>[2x]MKKQKRTQGKQNTKQIKQEKLSSKRKANNQKEGKKKVKQEDYKEIKQKGKRMLSKIVKASFSSKGFNLANAVNTVKSTLNAPIKHIKRNIEPTGSNYSRMTNTTEEAFDEVSHEWQALVTSNPFDLNVFNYLENTQTSNFGTVDNPLVVFTSETPFRYVGCTGQMNEDDYEGHELLFFLLREGSLQRCMGCGQVFKLVRLRNEYSPEMDYYLSNFHPYEMQEMGESDTTVLMSPYKYASHYEYTQFETPSNMVYSMVNPDEHDRLLVDPAYRMERTKALEEKYKVYTSSLREVEKQFEERYGRAGQINISKVTYSTLIDVEKAVLKMDRLFRKVAKFENRAFIDRANHSRREKRMLERAQQRWDSNYSFFTGSLTEEEQKYRDYYETELEAYPEDEGIEQQLDQQEVLLSGRYDPKLYDFQEGYTKNPEDDQTSLIEKKAFKFRYRLANETSETFQRRNNRMVERQIKRFQQPQYKHAFEQLQKNIAISSNSGNALHSEYGYLELLSNESVQLYKDYYESDAEEDFKVFENLSSKEKLVMIANFENNLLPKYDRSEVHLIPKRQWEPAFGVWENFLYDITEYASFIAPRGKEIAADYQIQSAIPLTKEELIEAGLYKETIEKKVEPKLEAKKQTKSE;>MIWKYLQRTNRGNIIQAGLQHRKFENLPFKQNFDNLTKAYDLRMWYISNSPHEAKNLEYVNELEALHNELNYQNSRQFLFRTVSFLLGWALFYQFYELPKTYDWQDTQEPKHQVPAYGDLEEGGDEGGDD[2x];>MSSAVEKKDLPADYGKMPAGYNFLTRGKDWREYDKDFILRTDAVWEKFQLEHFFRNYMKCFFFDHGLKKYQMFEPEDMYTVVFEGWALDDLITFPGFTPTGRTNSYQIGLSPRQRTVVPTQTFYQMQDYYMLCGLRFERWFRCDLVYHDQRHTKFDQVKNQKNYKTYPCYREYYEAQYACQDDMFDFLMELAYARRAADNFESDFASHELTTLPTFYDTPKAAERKTYTY[2x];>MGSVWFRNRYWWYRSLYDDYVAREAKLAFGIAAFIWLPHYYWGIHLNRAFEVNFSHRNYAHEWGPRRNRLAHSLEFEQFDMILENWQDLEDEYAQRGDGMLKK[2x];>MEVKYRGPSDDKLECEFLENNLLSCLREKSVQDNVAKMTCRPEFLVWFFLECPTKAAVYHDPKGLRNIFIQDKIKQKGSDDGVLSKDD[2x];>[2x]MNRFFKVSSKYQYYKYLEQYDAAFLRKYQSETHWYLGRRGAWKNLVIKYAGDHISLEEEHNVKYKTHLSFVYLSYRLAWVLFAYVLIYNHFLLGDIGKTFNVGEWDHRLKPSAERDYPTRYESLYILDRTQKW;>MISKYRYLHCARKLVKQSVQAFGGGHHHHEYDWRDDPKVNKDIEEDIRDRGWHPETYDFPYTKKHDDWVFDVTMPSQNYQTDLTVNIHPENKKMHVMKQVMRQSYWDAEHDMAHEYDYESEDLDFQCESFKSQHFRKKGPISQYLILGLLPILYFGTEFFYNHYPDEDYWRVAHPPPLDYPDTDDTDDTETFKDYKSFTGRRMVDTGIVDPLWYDIREGKKVYYDWAGVNQPMEDI[2x];>MNKSQDEVKEDYFSIKKKKYNSLDCVLSPIVTRKKQESINSFQAGLQEDQNSTAVPESPFIRNCSETLNRSQHKILDHYFEYDYSLKKKIEKIKISLQNKTGTDSSQSLVQKRLDDLRKKTLIYKQFNIQKNNNNINNTGQFFIEKDKQNNLNLSQPHQIIKSKQGHKRSFTNTLYCSSNDKKIFNISSQKQNIKTVKQSNNSSMYEEQIKNDQNKKQNFNKQAKSERKQAEFCDLFYESMQKDAERQFKSNSDKSKSITQILENNCENAIVLLNHLIQILTDSIPISKNSILLDEKLSQCVNLSNNSKISQLMLVIQKLQGKISYYYNDFLKCIRMMKICKNFCQLFGTLKFKISCYKYIGLGFQRLNKPKVALVYFVKMLRQSWFLKQEDQEINSYDFIGMSYFYLGSIDKAYQYHQMMIDGIKADEEVKKISNIMLKNRKYSNYPTLQNIRIIQETSDGQPLQKTIRKSKIINPQFQLTQQEWGENISSSEDEFELPQMQIAVKNAEEQTFQKKFLSTPWNDRFIQAQIHKLEIAQELNYNKFPIGLVFKNQSVLNFPNSSNQPQLVVGPYANKIYNQELSSTYSSRQRISHQTPNREFFNYHSQLQQVKEQTQLNQMKQQYNQIVDSIELANHLIVLKNLKKVKDLFQNLIPYLNEKYYNIKQQNTKSLKQQQNSFDAQNSNQSFLGLQNYSIQINGILNINNQTDEYVNNQSDRSYQQQSDKLKLLIKSKSRNHSKEINMTQNYFKSPSNESKQIKNLRVIVDNSNKKKAQQKLNQEFSMNFCESPKYDNSILSLFINKLSQESALRLEIRQIGSASRYQRKKQQKGKQRKEKYQKKQEENKLNIKQYKKERYNMALFFMANTAISVPSVLDTSPCMKQMLAYEDCVLDANVPQQEVIHPQWPTIWPRLLTDGKLLEFDKVPFHPENIYNYTYMRPLTKKNKQYLYECEEERFVFKACLRKVISLKKTDKHTSWDTAEVANLQLT[2x];>MLSKVTRRFLNYNQIYCFASQHGAEHHKLTASDEAYLNEVRQRYVTPDMEKWAYLDYKKHPSTTLSHYDHKSKDYVESERDDYNADVATNSHNKLIDDFKRNLQMQRKVHDILQKMDRPYLRGVPGVTKNISAGLQDYSAPVSKKSQSDPNDFYRDAYRNENRWIDQSVFTPKTSKMTHYDVEWPKELASRPVTKKFHHDKGYKYDVTTPYDQRYNYVADRLGHPEILGNPFERLMRLEGDIYHPNYLDQPFVKVPNANPNASLNFEEGEVLYENTRLLEWAKFWNYSVVVGYLWCAYFVPYNIFFKTHMPLEHAYDNLFFPYFQHTHFLWDNNALHIPTVGGVAIYATYIALSYINNIWKDYVVRAQFSKDKELLFVTRVSPFGTTEEEVYEVAHLEHLPPSVRSGVKDLSAQDADGLVDVTCMSSQRSLVFYKGDQYWNPKVYNDFINQTSNLWTRNYTGYNRLEVQNSVEQVKIGFSHSSQPKLEKK[2x];>[2x]MMQNLKKFMSKTIQVQPVSFNQIPKAFYNFPEYRTGGVQANPGITAKRIIKCIGERLRKYDPARWENVPITFKTHFRDENGYSDVATSIQIHDALEREFGIDIKDRLALVTDVETAFYIVMSHHDPL;>MFRRIISNGALLSTQTQRWQDLSKFACLRASLNKESEKAFQELAKKNNVSPQELVELSKIVSMNLDVLKQNINSEQFLLEKESTLKRYRQSSIGTRGHLQTVNEAVNTKYPTLAEGLGQVAGYKEAYQALREIFVHPSISVNNLRQGSYGQQFAVDFRTRADEYVKALLKDHSSNPQAVQTIQEIQHTLHQIIKNYEQNPASIYARILTVLQTRGVNTLPVSKTADQKAVATIQKTSTPSLTIDQLTVPVQERVQTQTVFDAELAFIKEANEMIQQNTGNLPWDGGKKKIFQGQANKYLETPYYLLAALSGLGLLYFLYSGDAKYKTLVLTPVVGIAAFVLLRRNQILNRVPTLTELFLHKDGKFVDAVVSVNGQLISKNDIPVSTLKLYRGDHTVKVNLNDFEDASAKKFLAQQSGQEGVINVHFSKLRNLAARNGQVLNLGDTEVVVPFENQANRIILKQIFKGVEVLPSS[2x];>GNLYTWGQYASGTGFETASAVPRKVDYFSGNVSKVAMGPYHTAVITNDGSLYTFGWGQNGALGNGAKEFQLSPSPVSFFNDKKLKVKDVVVGESYTIAVTENGEVYSWGYGGEPSSKINLDFFRNAILPQRCGALGSGDNKNRLTPQQIANLKADGYKNISGGDNFATLVNQSGEVINWGTGLFGSLGNGSDYPLFTPEVNAYFKHLKEHEGLTVQSIKSAGHFSAALLSNGKLYTFGVNTQGQLGIRENLGHNTDQNARLPTPVVDRHFVGQKVVDFEVGENTLVFLTDKNEVFFSGLELAYQPIRWEIPTDKKIVKLAASKDTFAAVTETGKIYQFNEFVGVSTNEVGNDYNVADSKAFEGKVVDLGGSYGIRFAIVN[2x];>[2x]MSVPSLEYQKQYIYSMQKSQCSIQNQSINIIADEQQAPQESYLSRKCQRHLFETKCVQLELGLNGDYSLSNNSLFIQNNNTVFDNLQQNTESNIKQTNRSNKERYETQIFEQHPIIKNPKNDQVSSIMNEQEQKKFINTDENVQQTAQVSKNSKQSFKNGIQQVQTLSIDKSQASIREQKKISDCNLDKQFIKGDSRLDESSKIPSKCCGWIPEDIIFENNIHQLNKKVTLVAKNNFSDSKIQNHKEKKYQQNFQKAAEIVNRLLNTSMNRIMRVRQHVRNFIMLLKLRYLNRKIDDLTDRDYASINDLSNFYKSHKKKRNSKAFMKHFNFVIKLSQKLPIFMPTDTLRVVWDVILVLFTYIFLYFYSILMFFNQDNPDTEFIKEFYFCTFFIFLIDVLVNFNTAFFNKDLIIINRRQIAKQYIFSTVFFTDFVSLIVLGIKVIKRSNFIVYNPNHNLLTYCFNMLIFFKVNGISSKKKGFDYVFTLKESEKHVIKLINQLFSVITVAHLAAIGWYFLGILQVVNDNQTNWLVKLNISEGVYYQKYIYSIYWSITTMTTVGYGDISATNYGEALYISIVMLLFSCVFAYSINNIGFILQEIEKSSKQLNDKITTMQRYLNRKKVNISLKSRIRHYLSFLAQEQRDRDKQAEDEIISILSNKLREEITVEINSKILNKFNIFSSNFSKQTLDKLVFKMTEVLINPNEIIFREEQNDDMSIYFIQSGVIEVYQQSVQKQDKVTVIQTLTDESLFGEISFFSGLSRKASARSINLSTLYKISREDFIYIIQENNEDYERFKMIQEQIVFQGELPLLHVECYNCKKIGHISSSCPKTHQIFDKQFIILREIYSSFQQRIFFDRTRYKNNLKPLNLIQDNQNVCKILKQNLQDDNISIEIMFDSCNRYTGSSYYNSEDLEDDEYGQCDEYATSSNSQTNIDNFSNKSSLNNIKNNALQKKKTMKKKEVSKKYLDNNQICENISSILNSDQYCNSQKVISNNINDNLEIKKSYVKSFNLSNRQKSLDDFEKIKSSQNLEQNNNFNNSDIQHSKSQIQIKADSEQFQQNIKAYSQTNKNEVDGDQEQSNISQIFKKRKSQKQQEQINNTNTDIKLQTEYPKQQARFSSTSGSTLQSQQLKMPSQKVQDELQLNINQNLKGQEFNINQSNKRVSTLLNQISNNHNQILKNCTEQTNYRNSIDQILLQGILVNNLIQSHSSQNILPIEQSFKYLKKADGDLEKKKNSILLQNFSLNNNKSSINITKEFIEDQAAVSHKNLSQIKTKQSIGKSSILNALSNINNIDGNTNDLNNKNNNSKLLQAQNSQITNGNQLQIVDRLSKLLLNPQLPLLLKLTSVGMSFREMNSINSNNAMDMFDKMHNFKKFFPHNNIENVLNKLKLLQLELKKQKKQKQINKPRRQNILFFRYYSNCGSQVHDNLKLLQQEFNIDDYRPTYLSYGVSKRRGQQFPCNKHNLTLYF;>[2x]MWVDFIDQTKSLKVSVNNYFYYLDRIKKLFTYLNDLRKHILKKYVYTINHKRIAINYLYFSMVTGLSGAALATMIRLELAHPGSPFFKGDSLRYLQVVTAHGLIMVFFVVVPILFGGFANFLIPYHVGSKDVAYPRLNSIGFWIQPCGYILLAKIGFLRPQFWRYYDKTSFSFPFLEKMKYNQYKEYKNDYLFYLDFLKKEITDDHSFFWKARKVIKLPQYSVFSFVPLKLMMWKTMINYPESFWYAASRVVQSRRKKVFVTKCSARTLTTAGWTFITPFSSNIKYTGVGSQDILILSVVFAGISTTISFTNLLITRRTLAMPGLRHRRVLMPFVTISIFLTLRMLATITPVLGAAVIMMAFDRHWQTTFFEYAYGGDPILSQHLFWFFGHPEVYVLIIPTFGFINMIVPHNNTRRVASKHHMIWAIYVMAYMGYLVWGHHMYLVGLDHRSRTMYSTITIMISMPATIKVVNWTLSLVNGALKIDLPFLFSMSFLLLFLVAGFTGMWLSHVSLNVSMHDTFYVVAHFHIMLSGAAMTGIFSGIYYYFNALFGVKYSRMFGYMHLIYYSGGQWVAFVPLFYLGFSGMPRRIHDYPVVFMGWHSMSTTGHFITLVGIIFFFLMMFDSHIERRASTSTTLGLPRWYKRISYYIFKIRYLQHTKSKMNGIPGSTVRLMLINRHFVEYEVYEK;>[2x]MWGNLWTEASYQLNFNIGFSSLRSDVLIHLAQWQYWWWFWFALIWSFYYFIILKVARFRVLKMRPKISTSYRPHGKWGDFLACIIPLIWCINILTNSNLILRLIEWQNESSLFTVRVRARQWYWIYKFELKNFTDILSTPKNIGNNRWQINTFGELQTADDYLHVLQLRSQNKWVKNYWNRSLQETGKTNKAHVISPQEQLRLSLINQYKSLNLSSSIKHNAPFINRDLYVFDDLFSYNLGDITTKKSLFNDKNSFLTSYSYLNNNSWNNNEFDLIDNLPFTTLFDNNDLFNNYKSFFQDSIFNSPKKQLSSDSKQLFKHIIYRSIKNNIIQDYTKLVKHEDFDEYSRWIKRSPGEVLPLRIIKYPLGLETIHNNIFENTNNEGNVELFRLRFNSNSSKMQHKLVQDTIYLTLKQKRYNRKKVVAPQIKYYKDDNGNKTDLVKYTGKPYLSNDKLLKQSIYDQTTQYKLIKKNKKRGELIPVTLARRILRTKKTLVLPAHVNITLITNSYDIVHSWFIPGLGIKLDCVPGRSTHHTFFIDNVGFYYGQCAEICGRYHHHMPIRVCALPFEHFLLWWNTFGLPKMLNTVSRKRFETHYELRKYSW;>MLICNFLMYSNFSRIYWFDFNGTVNENLPLNYNVLKICRNEINKLEKLNENNLGTQKNPIKLNLSFEDKHYNTNNLVLDLNSYETFNSKNFISSIFDKTFESLNTVLMAPIYSFLEFKLKLSSTKINTNHYYVINGKLYITYNDSFKLFTTINDYFNDLNELSNTKLFFLYRSFNIYNIKLNSLVDFVFLKLILFIHLLYLKSTNYNRFDYRLKQTDWGFYINNNSNYIQNIFSGLKYIWRGLRFWIIGLLLGLSSIYYLMYVRLLPFNKIIFAWILVAMFLYWLLSGFVFFVKKYQYSKFTAAIQRFWKRTYIIFWVIEAGTFSVFFYLTLNASSEPVYMYDQIKIYKTHLFSWRWFLIKLLPSVSIILLGYYLQLTLKWNLFNKQNTIVLLITLLLLYILWLEFYQFYHILSFYGNINWAFDYDEYIWTLELDTRRTRLANNYIAICLFAKFWHFVFIFLFWVFFVLRINELGRIRYPLLVANVQNFIIIYIMSWAYMYPWLKFIFRKYLDVPYYWFYLNGRELGIRVFFTDLKLFFYGITNRLFDFNPSSIKFEKYPFYYWINSSQLTEFNQYRKFVIRDSIIYSLNNYII[2x];>[2x]MYEGRWKMVNQIKQDVQNDIELILRQMNERIHAMKKKKYNELKGKIKQKCIDLLIDYAKQKIGKKNKIKKEGNNIRHNKQKKLKNIQKKIFKIISTRMLQTTLSAFRPRGSNVTGKVALATLGALTGYGAFYHYNQYLNLSARWQQIQENIAKDQPFDVDGFDAKVYPWVRENNVNDWEYKLVKMRGYFKDQRFFVRRKRDGKEGFLVFAPFVTAVERVNHRLKQKDLLPVEYSVFVNLGWVPVENKKDVELGGEVCPPMDAPTDSTLFVNDTFTGFNPDPANPEDTEQVTLTEITGIVRRGEQQDILARRRNWNKEGIYNWVDLDYMGKIFRLFNLDAINTAYIERVVPSFEEGEEGLYPIPATKDTFERPLNTPERHSTFFNFYAATSALSFISMLLLRR;>MISARAVHRFLRNPNLETGAAFRAGTRFDPFKNTLTVLKDPQNGRTLYLIGTTNSSTLLANRTKDLVQKEKPDAVFVQTNKEWWNLAKNIQDVKCQQELNRYNDLLSQAYTLSLDNTIRNLVFKAKFYSWLFVINWFKAFPDDFHPFIPGLEMKFAIEEANKQNIPVVLGGLEVDDVTLSALKVEPRLDPFSQLYYGYRALHNSFWRREHFDNYATLDVVGGEAYAESMDRFRTNWFVKYFEKLAPYQKKIIVDQKDLDLFYALYRDTPGKKIVAVVNQWHVPGIENHWKSATNTHEPLKAINPIGDMDINKYMESQLVNDTLRAFVSKVGKTEPATWKNYSTIYHKDNYEAERVRHVAFVDHKDPHMYHGLPQDYDDNIKPKHH[2x];>MRYLKIEKEKLVSCKKQEQEVQRIRRRKGNQKLNSIAKQQRVKRRDYQQNIKQNKEVKNPKKLIKQQIINKVKKRKKMFRGLTKFNKVFALNSFKNSLVAVPKANLNHVQNMLEENLKYDAQKYNDEVAVIQKTSRIYKPTYTIEFNREGEVLVYSADPIKNSVVYFKYPYVLYEAAIPLFIWAWIYNPLELSKNAVNSLLIYPNIAWIPRMWYWRSLQYKIQKMYLLRGGKVAKIETQSLAGDRFTSWVETYQFHPLTQDQKNFDNQDNAEFLEDEGQLKYELGVQLDNLQEMGTTSQDIVINFMKEGTVHHPELFEAIVKGYNIDTSDYVINTANNLRAREGNHNH[2x];>MSAILKRAAKYKRVSSILCEGEAHLRDPFTPPPVILKPPAPRKDKKPDDITDFPAQKLIPLPESIPYQEGKYRPASIPMVAGFFPYNCYLQQGKVYSWCSCGISQSGPWCDGLCNSVVTRCRPVVFNVSQSGYYKICNCKFSANAPFCNNTHRKMVRYHHQTHRGFYEIWGAALFVLGWVYMGFNYYT[2x];>[2x]MFLNRLVKETSKAKRLFSMAQNNFARAGPYNPNRYKDYYIPRTLPKNEEIVEFVQSQHSVPASPIRNQRHINPVRESGPLPSYDGTYTMEDIRAVFYNTTVGRDYCYCQMDPEEIMRRVPGITRKEAEFITKLGLSPQEQVDFAYIAYNIGLDIFYFTNQMFVARQVVTNSKGEKVEVLWNAQCYEDIAQLNVGFAPVLESVDYHWEIFLWADPPIKPNNDFDLNVPCTWFEYEQEWWMESCIQEDQFNLPEDERPYNTPRNPHCRKELWRSQDALQEEELMVNENWYPKNTQYNIYNQPDFIKPKSGSGAAADDIRI;>[2x]MLQQVFGKSKGGEVTNSHLTPKVLNKAQEAEKLASQIQAQRFSNRLVAFSSQYPRAKLFFAGIGIGTLLYGANQSSKARENKVATETRKERMAKPTIQLTGADSQNPPFTEKNINDWLYKTVSITGRPIHGKGMMIPAKSYGLHGFEYLVPFVTKENEDGSVQEGLILNLGFIPREYAPIWARARVENVEEQTFTCVVTDGKHLSEQGGLFASNKPCENQWEYADLDQLAKHTGFVNQEQVRSCILEHVNTETPNDERDCRHIDICSDYKEDYPYKFTRSGVLQQPGQMYWDLNKSASYYSLLGLGCSVFSALLFLAK;>[2x]MVYHLFERICNPDNFKLSGEAARVRTLIAAGFSKEEAEQVAWLQNHQVNGKILGLFTGGFALYCCNNYFHYFERYFPRLRYQPFTKFLAQAATVYFFFKIGDYYFTSRRYGSNDARMNGLMYSNTYYSTNKEALIQNFEPLNRKFTEEEVEQFLRNEGRSQEEKRNWIYNPHIHGSTEGEWKADIHEKFDSGKAPWEREHVKAKILETNKAKIDAGEEIQLKPFKTLNHLDKTGLLHRLHPFIWTNNWTLLG;>MSSFIQYEFLKIYQGNQKIKNYYKRKRLIFQQKKVLKKKQKEIQMSTNNLRLKPWFHWTDEERSHAIFSAYEKRILKSEDLPSFLRANRINNVSTWVFPLIALPLFNQSIFKLGFAQRILLTRPAIEWHCFKIATVAASWLAWLNFSPFYRKLENEKEYLLDTLESRIGINVLDLNDALPRWTTSQEYNRRTQQLYNQRNGFFAGLLYPQEESSRPLVDIASFPKNLHKEKLTK[2x];>MFGRLVLKQTRRTLFNPVLKNTFCIYQAYQNPLRHINTGHNPNNVYEDIVMLGDYPVQNRTHDKVISQTYVPAIANIAFTHLSKKYPQAGLKVDQLNTLKEKTWNDLGVNIEHEKQEILVELSEQIFVKESKLRWVHEQRQRLAHTTYVFSGLEFQNVKVGFFIDSYNFLLQELAHRSNLYQSKDIVGEKSFHEKHLEQQTAPYSGVKSLEEPVSQNKSFINSLMRAIHNH[2x];>IKGNQKKQKGKNQSNNNNNIREEGKQIKEMILPHNNRQLARQYFDSLPENDINRKYYEGLKYETPKTFFGRFLNQFNIDAKLDTLSKFYTYQKTIRATQAELQEDRKSYLTNSLLFTAVSWFSIYQFARKGAVLPVLREYGRYFGTHRLFRQYLHTLVLPLLYTEYALNQKYYTHMEHLWTVHVNRLNQKILEDPLYTFYPQELNVPKHNIIVPTIFRDTPQ[2x];>MSLSLFGVKNNWHKNGIWWFSKILNKTVGEERYDALRVQRRIWSMRFYYARQQCLYELFVDHPDLAQWTGTYPKVDSSHGFPFYSTYEMYRDFQENTLNSDGSFAQWITLVCGIYVIHVIYNYMIPYYWVSTPLKNDEFTRLRMKDYIASTVLEEVYGISYAEWGWLPHDFAYNRMRGLAGYMHPDDPRAMCTSTFHRKHKYIEHEVEKVGDYHHMTYPK[2x];>MFFELEDIKRRHSLYWDIYNVQGWVRRPDSTLYNNVKRGVTAGVVASLVQENITALVENCKLLATKYEKPQNLRQAATFMKEVFKLENYRKAVWNRSQYALCIGTFDIGARLATFRWLNNGWQRVFAGFEFNFVRKIPTTMLAALFTAPFSVPFELARMAYYGDKTFPKELQRGYSSYLSALARIPFEEGPYFLFKNSFPLIIRNFFQTFTLFYTYDFLKDKASFAWRVGEQNEYACKMIIAGISTYLAAVFSYPWMVTREMVDFWPKVPGAPCTFNGNYRKAAVWIWYHEFSGNYFAGFFTKYFWKASPGMFLTLMLADKVGLFDQTTVDNFGGAGNNSWEDTFV[2x];>[2x]MNYSYKRYWEPSTAEVIGLSLSVNTISAALTYPIEFVKVRSQIRTEGVGIRSKNLYMGINPNKVFREIHATGNGLRGFYQGFESHLIGRLSYLFIRNLTYKIIYDRTKPVKAHNDLSHREKGVIAGFAGGLAAFLTSPADLVNTRTIAEGGKPKEWRWGYKGLMDGINKIAATEGGNAALFRGSYANVLRAVILNISLTGPFDYLNEKIWITFGDMTWNKYAALLWASFWGSVATLPFDNIRTRLYAQNADPTKNRLTYSGWADAAKKLIQHEGISGFYVGFYAFYIRTFLYAWTTVFITDKITSDWKRKAGLKEWQI;>MANFVIPYLKPVADFWNSLCIDQHQDSLFQFKGQTGSLGTDWTSKYLRSEQDVYNHKYLQYHKRVHEAPELTDVISDNVYRLTLFAGVERVLSVRQAQAILKTQFAGATENISGAFQTVLNGGIFRRGYFRGALLNLLQFCGAPYQSLIWSRNSGITNQVIVSSIFEAFFYPLDTVKTLIYNDVQGKYKGAFHCASQVVQNAGWSRLYAGIFQKLIFNSALIFHLNQVWDGSSQQWASLALVAAAYPLLVLKTRFQVAGTPLALATSNEVLKVNRKTLYAGLVPYLIFNTLFAYEFAAWHSSTAQERVIGGLQNAMKQFSSPAAEQVWSS[2x];>MKKGTASEEELKKLYDPNTFYEHGDNPAFKQFMNIAVENLREGKLTDHRTYVVDTYKKWMYARNWDDFLQRDCKAITFPRAFALWIVGTLGMATASKWCRQILPVGSHGITKISQTQFFHQFGPLGTLGAVGFYGLTAYLYYKTTIFTVKKFYSHCILQEREWIFEQERQNPGYGEYFFKDVPLSAEEHFNDLARGEMAKKKFEKPNHEF[2x];>[2x]MKEKIFNELTRKMKRKEISAKIQREENKQILIRQRNNKKYIQSIQGIQQERKKGKLYLVEMATQNVEEMDTIQKMNYEATVNMGRQDLITREYTFYSDYEFIPIQEDRKQQMEDALNNLHKIIHPTVTQLKKKANVQEIQDRVFRKLQGWEGELNTCVFSAKNVRDSNFCADRFTNRINTEGVEFVKQILREY;>[2x]MNNTFKFLHQVISKLTLKAQVPNYGQYSHSLKRPINPKVVVFGNSSRAYELISSQFRNFNHVNGLELKGQEDNIQANKVAQSVLSINDGFQDGYYITDFPQNSKQAERLDLITDGVNLALYIKDPSDKVTVTRQQEAIDYYRKTGALVEFEVDPRGDLEEQVKQLSNQVLNGYKH;>MDNNYHFWGNGDRQDVSLSYEDYYSILDCLLDEKLSPQGLMKFKNLHEVSMYGVSYVPLYCFPVAYGISHMLTGKVRRGHSGYRNLFSLMSVVLPFTCWYAYTTPIPRRLYTEIICSNNADGAYVRNRIKQQKPGIWRKLSQQLYNKNFRFPELNQDLTATEFPLDYVAPHKF[2x];>[2x]MVFEFLFYNQQHKTRNGYFINHDNLMLASLEERKKLIFYFIANQVPEKLDPVDRVKFNEELSDNLSTKARLIGSLTGLIGLVGFPYISTRIYSRPVLNIGLSLLICPFLYYVGNQLTYSVWEPKFIANNNTVCELSKKYNFTVFDFAQAKKEAHLKALRTELVSDNLLYSPGI;>MAIRNFVFKISNQIQNLAAKRSLAYLNQIDSQSVPSRATINMKDQVTQMQREIDNMANVIRAQIPDEDRAEFEILKKYYVTGQHDSLVDPQDVLLQLDRIQVLKNLKMIELNEEAYDPELVRLEKLKARVLLEEEGALLEYAHFISKRPYNKPYEKWGVSEEHVKQQILG[2x];>MGFETVVPAPPTRDDELRMIKATEEQFLQQPRYKLYMNEAHRIAKMNHGDRHNNIRAHFWSNFALGLLITGPIFIIPFGKAFRNLRSGVPYYFRPKYVFTQKNQYNQDRNWGAMKKQIPLWLGLSTAYAYWFTDFSINDDEWLEKGKVIYPHQTIKVL[2x];>[2x]MDTEVSNHNYTQAVAYLNRATSSCVKKCDSLNNNGSLSSKQESCLKTCAENHAIATKIHAEYIRKLAESKYL;>MSDKRKIQHEGIIALINYSTLCAQKCDVLKGHDDKITDTEEQCLRVCAEKIRQTFEFTNDIYLKNPNLTKPN[2x];>MSTRKIFDSEEQSFIRLVDKFYLGLSLTKLCAQSCNLLRNDISGSALTQKEKDCLSICYNNIEKTQSAFYAKVKTTMNLPAVEDDGEEGGDDE[2x];>MEQNTTQVFSDLAYKVCFKVINDKNKPFVLHDEQRLANCLTRYVEAFNVTSEYFFRERAGETKVTEKQ[2x];>MEDNYAADVQRQFNRTAFDSLYKICYNSLVQKNGSTIDFQKQIDCHQRLIQVFAKIAPIVVKVEQDAASSGGAAAGGEDEE[2x];>MDPVLGDVIATRIYKACFKHVYGKNMKAYSEKDEAKFDQCLTSYVESYKSVTNHFITYLGQLPKKGLSLDGS[2x];>[2x]MSCTTRRFIDEKEKLEYSRGYNQQELEASKLRKDFVKKYIVDFDTTLYKTQVERDWAYIAKREYRYEVQLKSIGYGG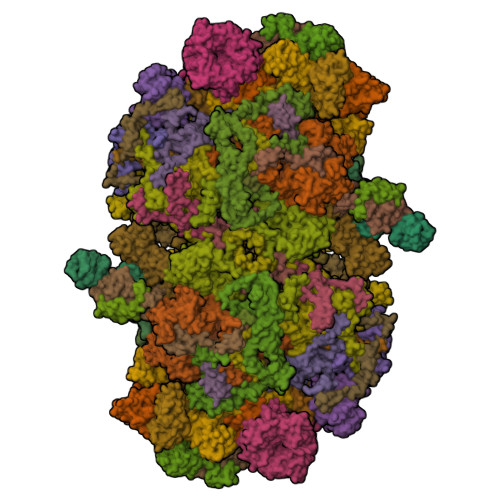ALANAVLLWRIYANKKMVFWPIPIVGALGYLYFQPVFFQKSNKRFFDMCNVGEEYYLGRERNKILRECNKILNVEDF;>MLIQIVLVLCQYFQLISCFCQGRLECLNPIQKRCVQIDGLQFIGREKKTGFCVIDSVLYDEIDFCLSESNNVCITYDRKMCIKVESNNSIVAINQEDSICGITIDGYCVDENQNYSQEIYCNDSHCKFTNKQYQKSCLNYKSPQIYGKANKNECVLQDQYFHSDAQIICKPHYCIYFQDKQITCVKMDHSIHPQIIGKDSDGICIFQKVEKQDFYLKYRNLQLCADQKHCYDTSQQTCMPLSASYPAVKMGGTCGNYNEPISISCFYEGNVCLLENPRVCIRIFFNQDYDVCGIRKDGLCAASNIYYQNLQICASDYCMYGQANNAKCIKMDGQQAVGIDSQGFCVQNFEQKADRCSTNFSYICYLNSSQICINLQGYQNYCQQANKCYEFSLQQYIGRDIYYYCIQSEQSLQPQNVQNCLQNPSYICQKRDGTMCVYYYQIPTYFTYLGYINSSGYCAQEGYQTYTSQPQFQTITNLNPNFCQDDSYVIQKILPPYYGRLDSYNYNRCLKQSDQSPYIESCIQGYCISNNSCQKIGFDSKNVSKLSNQYCGLVQQSSAIECAYDQDYCIYNSICYNLSDQNIQTSGIDYYGNCLQRGKYYQNWKKCSVNHCYQKKLLLNSFGCFYLDGTQGAAGIDSNGMCLDYGVSTPVRCALSSQVCLDFQKNTCQQTINFGSTGNGCYYSGYCYQINLGQFIGRDTSLICLSDQEATNNLDTCYNDNQNICMAVYSSLKFCVVYPRTSLYLGYIVQNKQCAVENQQTNQGQLVDLVNLRNNYCQDQQGYIRRLDGKQYVGVDSSQYLCLESGKTPSKSIIQCYTGFCIVENACKAYDQQYVGRDKYYQCLKKGEGISVECAANYCIDLSTKNCVQINDTNPAQAGVLDNFQCAHSERYYYSQILQCSESYCLQQNPNNPSQQGCFELDGDINRAGIDSKGNCLQQDLPNAVRCSPGQFCLNDKFGNACQSLLLSFKNNRFARQKGTGVCLSYIDPSQFKGDNIDICVKGSCKYSDPKNLDFCFSLGQLAFGNQVVGRDINGDCVLKDQQTSTQIVECFDMIYCILDLGGGKQKCQLLQEKDLQFPNLIYKAKNINQTCQDINMPNSMGCLYGLYCINPNDGYKCVLMNDDNKIGRSLVNQQCLQQGELIANYCQPDFCILNGACVPLSNKFPGKENQTQKCLPEQIEGQYGASNCYKEGFCLIINPQNQLASCYQLDYSNPNTIGIQIDTQHCLKEGETVAIMCAYEKYCIDPVSQSCKIQDIKQGYCLGKNGMCAKNGSCVYCQVSQCLTNQNSGTCIDLQQPPALFCKDINVHSENIFIQNQKGICQYLNSGQCDICPENYCKFNNMCFGSQDLLKILKGNQCFVYVPKLKTCQIQDLNTPNSQGNMNCMNNKGFCQDTTVVKNQCLMCANYYFNPGNQQCFSIEEKALLSSSQLFFNMQLIYVKQDCYDQDYCQSIPSLKCPKGCFSCNSPNFCTQCIEGFFLYQDTSNQQFCIQCQKQIIQDNTLKIYYNQIPTYSCLDCSSEYGTWNQISSKYRNCQNFIVKLDNLLQITSQKYAAQNYIISPISTTQAPYQLYFHRSRLCPTGCLSCVQISDSKVMCLQCQDYYINDDNGSCQKCPDFCINCQYATFISGKVIPKSQIEKNQQKYYYFVTICLKCSQYYLVSYNLQSCDNCGINCLYCQYENYKTVLNYNIRQLQYLSYYEFSTQNFIKKCIQCPQGYVVGYDGQFCQKEIQNCRYTTFQIAQSYDLTLYIWSFTQNSTIANQICKQCVDGYILSGDASSCLDGCQQQISDNRCESCYSPLNKIQCQFCNSGQILNQVVNPGACQDDICSRNIVGCQECYKYQDPQNPSPFYQIYQCTKCIDQYSIPSIFSCIQCPTGCAKCYEGYRYYNFTSELVYKRTQFTVNQRLNYYQNDYQLYCTECQKGYQFDQQQKKCIKIQCGPNCNLCILINNQPQCVQCNYDKLIAELNQLSYFIGILYFKQNYIPNPKTMISLTSSGNDCQICPILCETCVNNSDVSINPLFIYDAQCLSCKQSLDQSYVLQNYQITYDKSRRKCYLCNKSEQGCYYKKQKVIYAQCLDLSTRLGDGSLQNPINFSRLNEIDLNQFLINEIEYNQAIIYYNELQVKELEVQLIFVDGSCYDYRPQKFSINIKDSIRALSTSLNITTLNQNSVLKFYQLDAFTVQGFDQIYIKNIIFLQQRNDAKLGLILVDKALTNIQLFNCQFLQIQQLIQSIQFMTFNLQTIQQTKVKLEQVVFQNIQIFESTSLININNTQNSSIYLKMNQVKLNNVLFQQSKLISTNSMNITIDITNLFVNQSLFDQQSLLLDMKQNLLVDQYIGILLNNIIFLNSSFLHGSTILNSDFLDFLQIDNLTFNNCTFQQTQKQAVLPLIAANTFMLTQIQIISNTITNYSFLQQYDNYFKDQNQSSSFSGIDIIDNKVNSDSYLFLFFQTQQNRNSSIHGINILRNQFSSNYTQVIVQFNQQNFVQIQNLTIVDNQQFLFISTDSVRNILLQQVYQYQTSSQYFAAQICYLRQTKNQINIKNIKLEGIYFQKNIFQIENSLNNYLQKDFQITVTNLFSTQSTLLLKRYTNDVTIFSLYSKQQISLTVQNVTFSFFKSQVLNNKTSLGKISLGFYFQGLQIKATILNSTFADLDISSPFNWIEGSVQQMILKSCNFTNSNGYQNYNSVRNGGFFKITSQKLIIKKSIFINGNALNGGAFYLIMQGKGTLNLINSTFINNKAYSNNDQETKGGAFYLDGFMSESLDVLVFKSIFSKNLALFSGGAINIQSSNQQNAFIIQESFFFDNLSCQGSSINIQSSSDFQSEVVISKTKVNNQIQNTISTVENIANLLSQYTLLNIQQLSSSQIFIKDVRNVQFFQSRFQIVPYKFKDSNVLKYFKGIIFSQMFSIQNVLNYLDINNIYEKSVFYGKLINVNNVKNIQIQHTQILNNQNIIEDLSHQDNRVSNLASFHSQNCLVFNLTVNQNKCLQCNLGIIEILSSKLDMQNSTFQNNLAQYGSSLQLQQNKQYIYNLSKLLQSFQDKLVISNSTFSHNIANVNGGALYIKESTVFIYQTLFDTNTARQYGGALFLENTKKNILTNLINLQNCTFSNNKAKFGGVLASTTGQRVNKYTNNTYKDNKGYQYGENIQTSPTKFIITVNKTQLTDTQYINIQNHQGGTLRDEILLALCDDQNNYIQNIPQDSFLSINITQGSGFLNQNKIAHKNGIFNLTQQIQVYGYSKQQLLLSITSDLIQIPVFNKDEIIIGYDSYQLIINIQMVQVCLPGQIPKKFQEKFDLCYDCQDGSYSFQVSDTCQICPSPQAKCFRDKILLPSNLWRVSQKSIVLFPCKNCVGDIQLYKKFKKRSLLKIQSTDLNYYCKEGYIGALCEDCDRNGQHWGDSYFMNLDLKCQRCSQTTFAEIAYPLMISLIAFILMIFLTYYIQIQVHLKLTKKVLTILSKKYYGFNDQSIARTIKFLVYQSSIIGIMFWYDCYIPNTFSYIFIDIGNLFTDQIRISECFLEQKFSGTSIIYKGIYFLLGTYFAIISCIIIFYMLLRIKFNYQNYLQDILISLSIFVYFSYNSILSKIFRSVIHLLFLKIKKNVILQNITNRLIAKSLTKKDSQWSIYQFHVMK[2x];>MIQQMDQYISMQNESSSEISDIETRSPSHSFEDNLKYYSDIYEVLSKDQIKQEYEQLQKSNFVKNIIRSFYLFILESGDEIVIESMFENQEKGIIQIRKEFQTFTRQKKFNQSTLNSLINSKRFGKIFYYFLKYYIYDWVISRSVKDLKSHVIFITYLKKQLEQNIENQQFD[2x];>MGFIDLLKPAFSLIPEVQPARQYIPKDHKIVWTGITLFIYLVCCQIPLYGVVRAQGSDPFYWMRVILASNRGTLMELGISPLVTSSMIVQLLVNTRILDFNARVQDDRQAIQGAQKLLGLIMSMCEAFAYIWSGQYGDPNKIGLGSCLLIFIQLVFSGIVVLLLDDMLNKGYGLGSGISLFIATNICENIVWRSFSPITITTQQGTEFEGSIINLFHSLLTKDRVSNALYHSFYRTSAPNLVNLISTLLVFLVVIYLQGVKYDLRIARRQERNSESSYPIKLFYTSNYPIILQTALVSQIFFFSRILSSKFKNNFFVKLLGQWQDGSVAGGQDHPIGGFVYFLTAPRDLNQVISDPIHAIFYVLIILTLCGVISRYWIEFSDESTSSVHKKFMEEKIEIPGHRQDSVYRTLDRIIPTAATLGGICVGVLTIVADFLGAIGSGTGILLAVNIIYGYFEQVKKENKLKKTGIVQQQQQQM[2x];>MGKDQLDFSHFDKAFENKYDIVAPEFGDLHQKRAEFIAKNQGTYRPVPLVPNNIKGLIPKTCRLPATRNWYRRTSSFERNGFFNIHTPVLNTKMIPWLLFIVLTWGWSSFQIGGYNYERFDDNGERRNTLYWKLSPVEFPQSKLWNRPS[2x];>MVFHYTNFVQETNAWWLRRVRPVYCTVLAYYGWWLYDRYYLFGKNATQDIRKDTTEVWEKRAALNKRNWGYNAHYKPELERSMKKVLYADPNYKFPIEWPERYMAETKTLEQVMDEEENWEYYK[2x];>[2x]MEPFGTDERNWTHEEKDIITRFLKYDKHVNLKTAEMVYSAEVESAYFGKAGALAGGVISALFFNFPIVRNLPIIRRSVIGVLPFLYCYTWGKNTQEELRWLKTFAAYQRFVVYHGQHCKLWV;>[2x]MAQTAHQNRYQGGLCYAQCNELFSFWNPSIQQCWKGCDFGVGRVNDPEGRIEAQQMCKRWAAELYWTYKGELDTIKDLRVHADMYPTTPQNVYRACLAGVRRQKF;>[2x]MFRWLFLYWYNSTDTPSAIAKVNLWSYINLRLFKARLSSSIAYYILGLNNLELKKLKIFYKNTYFDYIYLKSIPCLFLIIFFTNLYLFL;>MFLGIFKDVIKLLNKKVVPVYFWFFLYCFLSTMDTNIFVSSCSFLKVEVFGKDENTTLVLLFYVFYSLFNFYLSRIKNKNNYLVRKHLYTTELLIELILFKYKLIILKFSSIKYILNFNVRKFILFNLFLINNYKAYKINTFFLYIYIYLNNLNIIWYPIFKAYSIFGYYKSTRLNFIDTKNENIKRIKY[2x];>MTALFLHILWSISYIIINILYIFLSLLLSNNNEKIKQYNSNYFIKILLVLFYNKNLSFYKNLLSEDEISKIEFERLKNYPTLVLIHSNLNKLEKRNKIINSFINFKTKYRFYKFISTNFNLQTIIKNCNDKIIFSTLLYIVNLNYSFFYKTIKNTDLIVYLLANKFSILNDNIIVSKFNISKFNDYIKYINNTNSIDTYLENQIILGLNNNTNSNITKNINTKLLNSYSNLKNLVNITNNTFYLKKINDNYNTVINSEFLTYLKSNYKISFSASNIVKYLSDKSVNNSVILYLRKNKIFNKSRYSRNRQTYRTGAYWCLYVNIIAVVAFYFWFYKFTMNFGYLWWLLYSLILSFFFSRALKHRFYNPLNVMTEFKNGFMWFIIILINIFKPLLKLLENNYINLYNHLVIKYYQSFICNTLINKKKLEFNYILSSFKFIKELNNIIIISLNKLF[2x];>MSSDPFKKVERDYHNERSVHKHFASYPLKFWWGLNKFETIQGIHSILGNAADLVVSTLSFIPGVQGRNNASYIENSIRVTRFRGFDDKTQ[2x]2-(methylsulfanyl)-5-(thiophen-2-ylmethyl)-1H-imidazol-4-ol 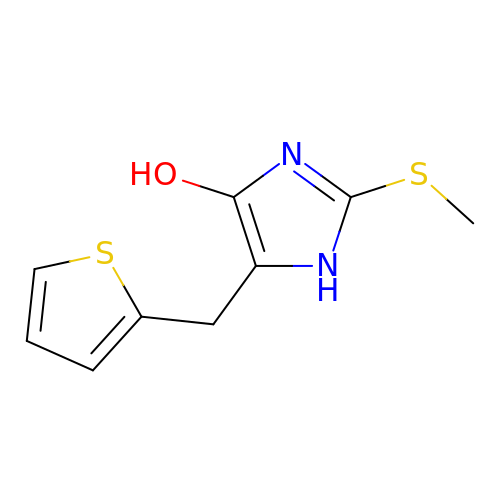| C9 H10 N2 O S2 | QWYGHJVEZLVLSU-UHFFFAOYSA-N>[2x]G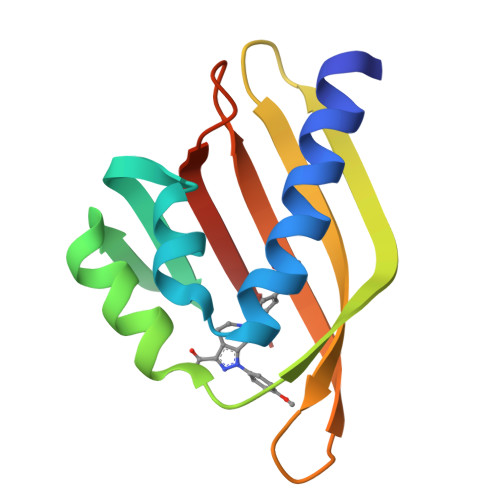SSARIAKAKKLIYKLEKLWNARDNDGILKLFKDDAVFNLNGVPYKGKEAIKKVLESAPKAKYKITKIDIKIVGNEIIVNVDVLATGPSGFTLKVKSTITFDEDMKITSYEVNLEGS>[4x]AQYEDGKQYTTLEKPVAGAPQVLAFFSFFCPHCYQFAEVLHISDNVKKKLPEGVKMTAYHVNFMGGDLGKDLTQAWAVAMALGVEDKVTVPLFEGVQKTQTIRSASDIRDVFINAGIKGEEYDAAWNSFVVKSLVAQQEKAAADVQLRGVPAMFVNGKYQLNPQGMDTSNMDVFVQQYADTVKYLSEKK

DsbA from E. coli K−12 (EcDsbA) was the first and is probably the best-characterised DSB enzyme to date. This 21 kDa periplasmic protein is a dithiol oxidase that catalyses disulphide bond formation between consecutive cysteines of unfolded polypeptides as they are translocated to the periplasm. EcDsbA consists of a canonical TRX domain, a hallmark of proteins involved in redox homeostasis, with an inserted helical domain. The TRX domain harbours the conserved active site CXXC (C30-P31-H32-C33 in EcDsbA) that is featured in many proteins of the TRX superfamily. The acidity of this groove originates from a cluster of negatively charged residues (E24, E37, E38, D44, E85, D86 and E94) that map along a buried channel in the interface between the TRX and helical domains of EcDsbA.

The other three mutants, E37A, E24A and E24A/E37A/K58A, were crystallised in space groups P21, P212121 and P2, respectively, with four molecules per asymmetric unit. The crystal structures of the three mutants containing the K58A mutation showed that the shorter alanine side chain at position 58 significantly expanded the size of the entrance to the buried channel. In all three crystal structures, a glycerol molecule, used for cryoprotection, was modelled into the electron density. The binding of glycerol displaced w2 in all three structures and hindered precise analysis of the water network in these mutants. However, examination of the three lysine mutant structures showed that w1 was strictly conserved, forming hydrogen bonds to the backbone amide of C33. When E37 was present in the protein structures, water w3 was observed to form a hydrogen bond with E37 in both K58A and E24A/K58A structures. Additional water molecules (labelled as w’ in Figure 4F–H) were modelled into the electron density in the buried channel in all the lysine mutants. Conversely, introduction of the three mutations, E24A/E37A/K58A, resulted in a less oxidising redox potential of −139 ± 1 mV, 14 mV lower than that of wildtype. Modification of all three charged residues (E24A/E37A/K58A) led to an oxidation rate constant of 5.93 ± 0.16 × 105 M−1 s−1, 3.8-fold (380%) slower than that of EcDsbA wildtype and the slowest among all mutants. Mutation of two or more of the E24, E37 and K58 further increased the “disordered” solvent content, reducing the structured hydrogen bond network between the charged residues and the w1–w4 water molecules. Indeed, both E24A/K58A and E24A/E37A/K58A mutants displayed significantly lower thiol oxidase activity compared to the wildtype protein (although the more reducing redox potential of the latter would also affect its oxidase activity).>METRTLEDWRALLEAEKTLDSGVYNKHDLLIVRGQGARVWDAEGNEYIDCVGGYGVANLGHGNPEVVEAVKRQAETLMAMPQTLPTPMRGEFYRTLTAILPPELNRVFPV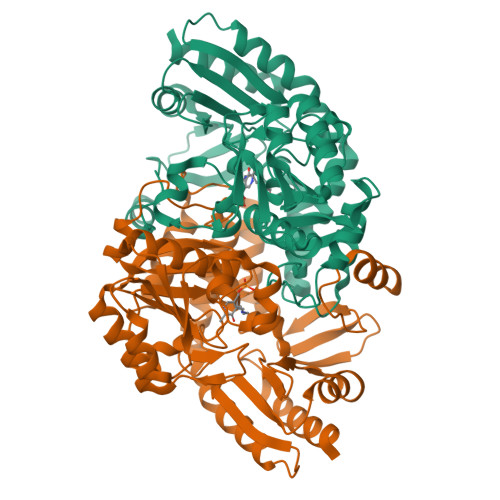NSGTEANEAALKFARAHTGRKKFVAAMRGFSGRTMGSLSVTWEPKYREPFLPLVEPVEFIPYNDVEALKRAVDEETAAVILEPVQGEGGVRPATPEFLRAAREITQEKGALLILDEIQTGMGRTGKRFAFEHFGIVPDILTLAKALGGGVPLGVAVMREEVARSMPKGGHGTTFGGNPLAMAAGVAAIRYLERTRLWERAAELGPWFMEKLRAIPSPKIREVRGMGLMVGLELKEKAAPYIARLEKEHRVLALQAGPTVIRFLPPLVIEKEDLERVVEAVRAVLA[2x]>AYTTFSQTKNDQLKEPMFFGQPVNVARYDQQKYDIFEKLIEKQLSFFFRPEEVDVSRDRIDYQALPEHEKHIFISNLKYQTLLESIQGRSPNVALLPLISIPELETWVETWA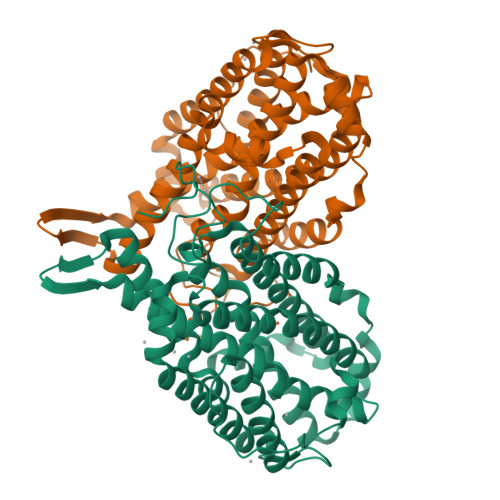FSETIHSRSYTHIIRNIVNDPSVVFDDIVTNEQIQKRAEGISSYYDELIEMTSYWHLLGEGTHTVNGKTVTVSLRELKKKLYLCLMSVNALEAIRFYVSFACSFAFAERELMEGNAKIIRLIARDEALHLTGTQHMLNLLRSGADDPEMAEIAEECKQECYDLFVQAAQQEKDWADYLFRDGSMIGLNKDILCQYVEYITNIRMQAVGLDLPFNTRSNPIPWINTWLVSDNVQVAPQEVEVSSYLVGQIDSEVDTDDLSNFQL[2x]PNGM-1 is derived from a metagenomic library from deep-sea sediments that predate the antibiotic era. PNGM-1 has both MBL and tRNase Z activities and is considered to be the evolutionary origin of B3 MBLs. The wild-type of PNGM-1 has two MBSs in its substrate-binding pocket, and each is occupied by a zinc ion. The zinc ion in the first MBS (Zn1) is coordinated by the residues His91, His93, His188, and Asp210; the zinc ion in the second MBS (Zn2), by Asp95, His96, His279, and Asp210.

His91 and His93 coordinate the zinc ion at Zn1, whereas His96 and His279 coordinate that at Zn2. In the structure of the H91A variant, the electron density for the zinc ion at Zn1 completely disappears compared to that in the wild-type structure, indicating the loss of the zinc ion in this variant. No electron density was observed for the zinc ion at Zn1 in the variant H91A. Among all the variants, H91A and H96A exhibit the lowest metal occupancy. From a structural viewpoint, the substitution of His91 and His96 by alanine markedly weakens the metal binding affinity for Zn1 and Zn2, respectively, compared to that of the wild-type and the remaining variants. The residues His91 and His96 are buried in the substrate-binding pocket of PNGM-1. In H96A, even though electron density exists for the zinc ion at Zn2, the density is weak and noisy, implying weak binding of the metal ion. Both H91 and H96 are located deep in the catalytic pocket of PNGM-1; thus, the substitution of a bulky His residue to a sterically smaller Ala residue could lower the overall stability of the MBS, in addition to the loss of one metal coordination. In the structures of all PNGM-1 variants, except in that of H96A, the electron density corresponding to the catalytic water remains despite the complete or partial loss of a zinc ion. Each MBS of PNGM-1 is formed by four metal-coordinating residues, and the substitution of only one of these residues dramatically reduces the metal binding affinity of the enzyme.

>AGGKVTSSTGIAPKRYVYYPGSEELGPDEIRVIACGTGMPTARRAQAAAAWVVELGNGDKFIVDIGSGSMANIQSLMIPANYLTKIFLTALHTDHWGDLVSMWAGGWTAGRTDPLEVWGPSGSREDMGTKYAVEHMLKAYNWDYMTRAVTINPRPGDINVHEFDYRALNEVVYQENGVTFRSWPCIHAGDGPVSFALEWNGYKVVFGGDTAPNIWYPEYAKGADLAIHECWMTSDQMMTKYNQPAQLALRINLDFHTSAQSFGQIMNMVQPRHAVAYHFFNDDDTRYDIYTGVRENYAGPLSMATDMMVWNITRDAVTERMAVSPDHAWDVAGPSEDLAPDRNRASEYTQYILDGRLNVDEANAHWKQEFMG[8x]>MTIKPAVRISDGNLIIKNRTILTGVPDNVITTSASEAGPVEGVFVGAVFNKEESKHIVPIGTLRNSRFMSCFRFKLWWMAQRMGEMGRDIPYETQFLLVESNDGSHLESDGANGVECNQKVYTVFLPLIEGSFRSCLQGNVNDEVELCLESGDVDTKRSSFTHSLYIHAGTDPFQTITDAIRTVKLHLNSFRQRHEKKLPGIVDYFGWCTWDAFYQEVTQEGVEAGLKSLAAGGTPPKFVIIDDGWQSVERDATVEAGDEKKESPIFRLTGIKENEKFKKKDDPNVGIKNIVKIAKEKHGLRYVYVWHAITGYWGGVRPGEEYGSVMKYPNMSKGVVENDPTWKTDVMTLQGLGLVSPKKVYKFYNELHSYLADAGVDGVKVAVQCVLETLGGGLGGRVELTRQFHQALDSSVAKNFPDNGCIACMSHNTDALYCSKQAAVIRASDDFYPRDPVSHTIHIASVAYNSVFLGEFMQPDWDMFHSVHPAAEYHASARAISGGPLYVSDSPGKHNFELLRKLVLPDGSILRARLPGRPTRDCLFADPARDGVSLLKIWNMNKYTGVLGVYNCQGAAW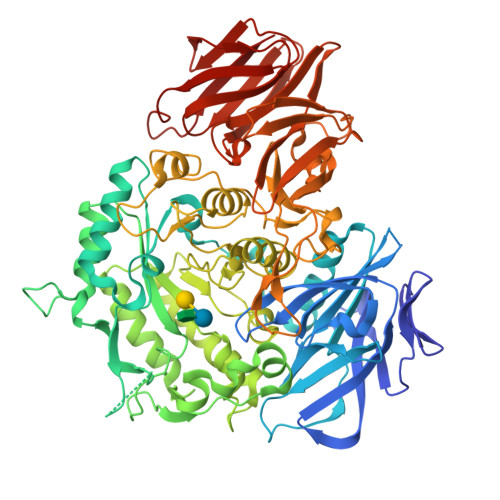SSTERKNIFHQTKTDSLTGSIRGRDVHSISEASTDPTTWNGDCAVYSQSRGELIVMPYNVSLPVSLKIREHEIFTVSPISHLVDGVSFAPIGLVNMYNSGGAIEGLRYEAEKMKVVMEVKGCGKFGSYSSVKPKRCVVESNEIAFEYDSSSGLVTFELDKMPIENKRFHLIQVEL[2x]> GSSST;> GLGQMLESMIDNTVRETVGAATSRDALPNTEASGPTHSKEIPALTAVETGATNPLVPSDTVQTRHVVQHRSRSESSIESFFARGACVTIMTVDNPASTTNKDKLFAVWKITYKDTVQLRRKLEFFTYSRFDMELTFVVTANFTETNNGHALNQVYQIMYVPPGAPVPEKWDDYTWQTSSNPSIFYTYGTAPARISVPYVGISNAYSHFYDGFSKVPLKDQSAALGDSLYGAASLNDFGILAVRVVNDHNPTKVTSKIRVYLKPKHIRVWCPRPPRAVAYYGPGVDYKDGTLTPLSTKDLTTY;> SPNIEACGYSDRVLQLTLGNSTITTQEAANSVVAYGRWPEYLRDSEANPVDQPTEPDVAACRFYTLDTVSWTKESRGWWWKLPDALRDMGLFGQNMYYHYLGRSGYTVHVQCNASKFHQGALGVFAVPEMCLAGDSNTTTMYTSYQNANPGEKGGTFTGTFTPDNNQTSPARRFCPVDYLLGNGTLLGNAFVFPHQIINLRTNNCATLVLPYVNSLSIDSMVKHNNWGIAILPLAPLNFASESSPEIPITLTIAPMCCEFNGLRNITLPRLQ;> GLPVMNTPGSNQYLTADNFQSPCALPEFDVTPPIDIP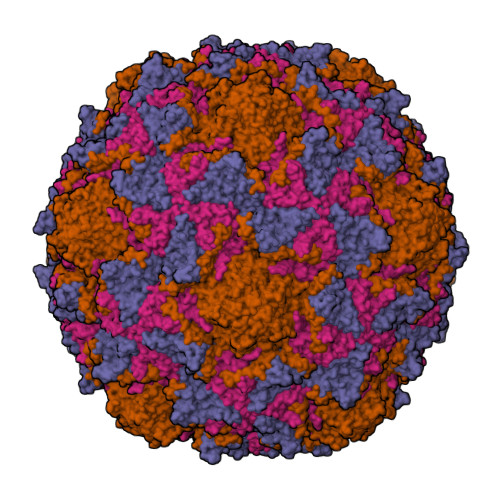GEVKNMMELAEIDTMIPFDLSATKKNTMEMYRVRLSDKPHTDDPILCLSLSPASDPRLSHTMLGEILNYYTHWAGSLKFTFLFCGSMMATGKLLVSYAPPGADPPKKRKEAMLGTHVIWDIGLQSSCTMVVPWISNTTYRQTIDDSFTEGGYISVFYQTRIVVPLSTPREMDILGFVSACNDFSVRLLRDTTHIEQKALAQ;> GAQVSSQKVGAHENSNRAYGGSTINYTTINYYRDSASNAASKQDFSQDPSKFTEPIKDVLIKTAPMLN>[6x]MLGLTLMFKRFFGAVRTSWRDPSTRGAVLSLAIIVTAATIFYTLAEKWSVIDSLFYAVSVGLPM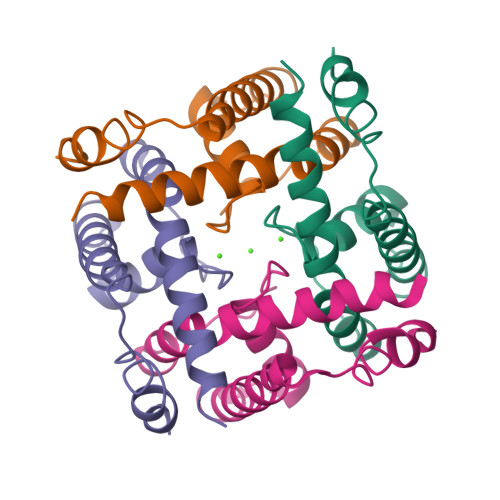GNGPLSPTLTLSKIFTLVYAILVVGLFVTVGGSLASAIVQNNTEKFKRLNRKGSAEAEDHHHHHH> GSTLDGPYQPTTFNLPIDYW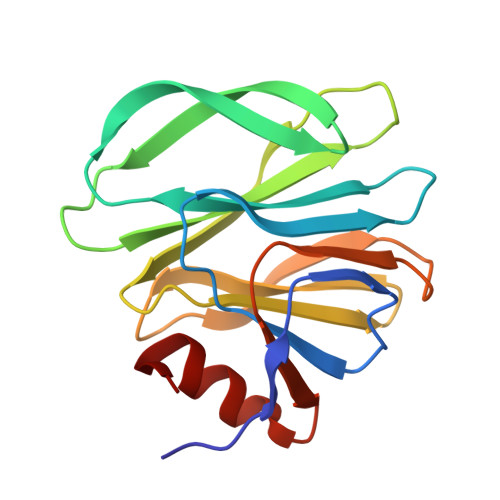MLIAPTQIGRVAEGTNTTDRWFACVLVEPNVQNTQREYVLDGQTVQLQVSNNSSTLWKFILFIKLEKNGAYSQYSTLSTSNKLCAWMKREGRVYWYAGTTPNASESYYLTINNDNSNVSCDAEFYLIPRSQTELCTQYINNGL>[20x]VQPLARDAMAYVLAGGRGSRLKELTDRRAKPAVYFGGKARIIDFALSNALNSGIRRIGVATQYKAHSLIRHLQRGWDFFRPERNESFDILPASQRVSETQWYEGTADAVYQNIDIIEPYAPEYMVILAGDHIYKMDYEYMLQQHVDSGADVTIGCLEVPRMEATG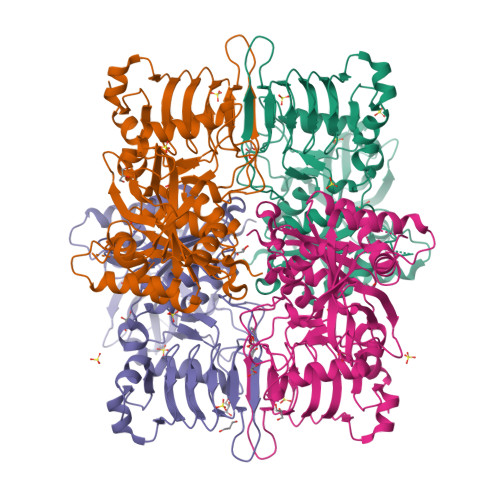FGVMHVNEKDEIIDFIEKPADPPGIPGNEGFALASMGIYVFHTKFLMEALRRDAADPTSSRDFGKDIIPYIVEHGKAVAHRFADSCVRSDFEHEPYWRDVGTIDAYWQANIDLTDVVPDLDIYDKSWPIWTYAEITPPAKFVHDDEDRRGSAVSSVVSGDCIISGAALNRSLLFTGVRANSYSRLENAVVLPSVKIGRHAQLSNVVIDHGVVIPEGLIVGEDPELDAKRFRRTESGICLITQSMIDKLDL2-(4-tert-butylphenyl)-5-[(quinolin-2-ylamino)methyl]-6H-[1,2,4]triazolo[1,5-a]pyrimidin-7-one | C25 H24 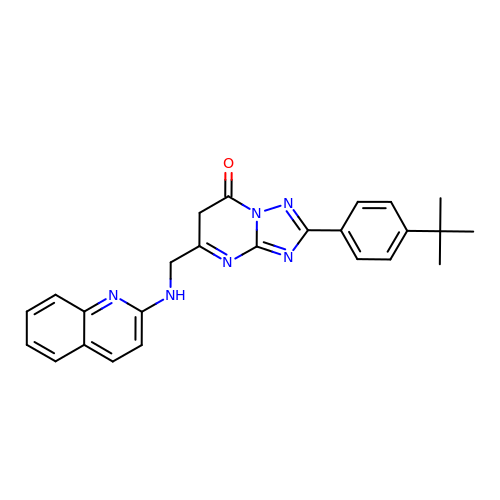N6 O | TZHVTFCKNRQYBM-UHFFFAOYSA-N> LGEMDDAPDENEALKRKIDAAKMPKEAKEKAEAELQKLKMMSPMSAEATVVRGYIDWMVQVPWNARSKVKKDLRQAQEILDTDHYGLERVKDRILEYLAVQSRVNKIKGPILCLVGPPGVGKTSLGQSIAKATGRKYVRMALGG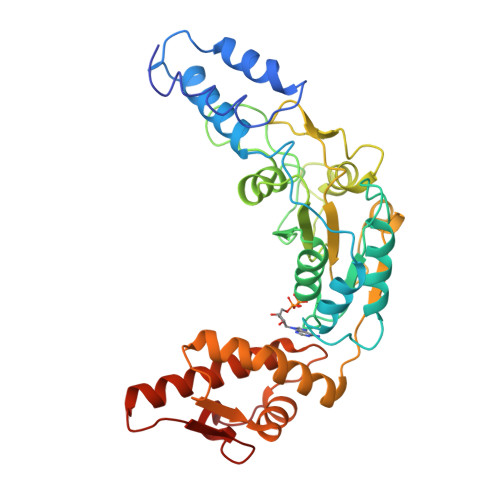VRDEAEIRGHRRTYIGSMPGKLIQKMAKVGVKNPLFLLDEIDKMSSDMRGDPASALLEVLDPEQNVAFSDHYLEVDYDLSDVMFVATSNSMNIPAPLLDRMEVIRLSGYTEDEKLNIAKRHLLPKQIERNALKKGELTVDDSAIIGIIRYYTREAGVRGLEREISKLCRKAVKQLLLDKSLKHIEINGDNLHDYLGVQRF> NLQNIIYNPVIPFVGTIPDQLDPGTLIVIRGHVPSDADRFQVDLQNGSSMKPRADVAFHFNPR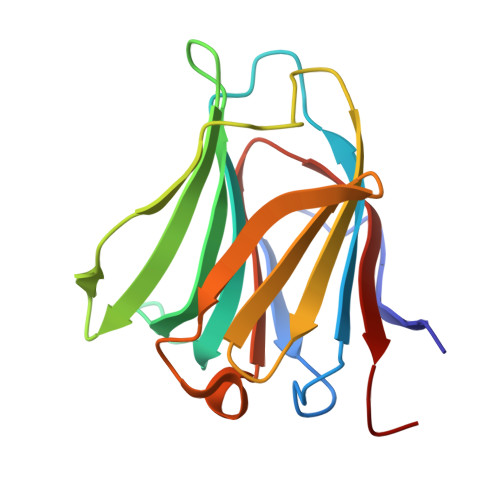FKRAGCIVCNTLINEKWGREEITYDTPFKREKSFEIVIMVLKDKFQVAVNGKHTLLYGHRIGPEKIDTLGIYGKVNIHSIGFSFSSD>[2x]LQALLPKAQSVGNSRVRFTTAEVDSAVARISQKIGVPASYYQFLIPIENFVVAGGF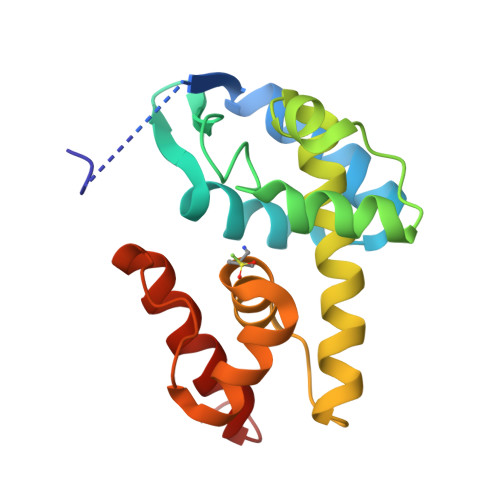ETTVSGSFRGLGQFNRQTWDGLRRLGRNLPAFEEGSAQLNASLYAIGFLYLENKRAYEASFKGRVFTHEIAYLYHNQGAPAAEQYLTSGRLVYPKQSEAAVAAVAAARNQHVKESWA>[4x]EGRHMQEILDAILSGDAASADYAALALPESYRAVTLHKGEERMFDGLASRDKDPRKSLHLDDVPLPELGPGEALVAVMASSVNYNTVWSSIFEPVSTFGFLERYGRLSPLTARHDLPYHVLGSDLAGVVLRTGAGVNAWKPGDEVVAHCLSVELESPDGHNDTMMDPEQRIWGFETNFGGLAQLALVKTNQLLPKPKHLTWEEAASPGLVNSTAYRQL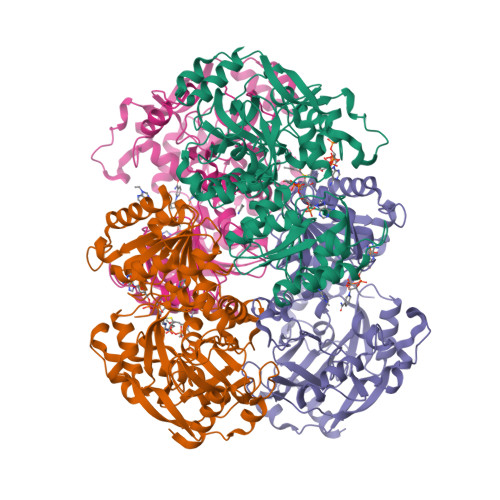VSRNGAGLKQGDNVLIWGASGGLGSYATQYALAGGATPICVVSSPRKADICRAMGAEAIIDRSAEGYRFWKDEHHQDPREWKRLGGKIREFTGGEDVDIVFEHPGRETFGASVYVTRKGGTIVTCASTSGYMHQYDNRYLWMSLKRIVGSHFANYREAFEANRLVAKGKIHPTLSKVYALEETGQAALDVHHNKHQGKVGVLCLAPREGLGVTDPELRSKHLTKINAFRN>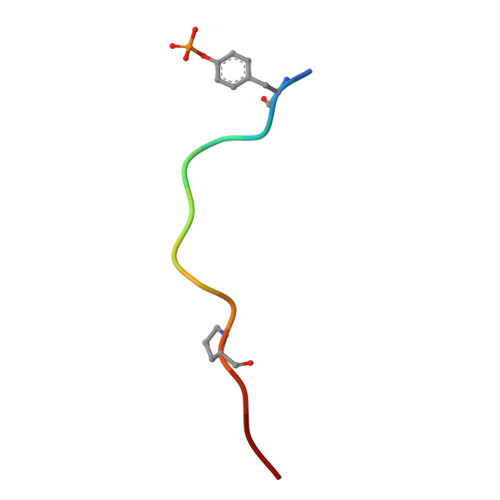 DYPKPSTRPPRHN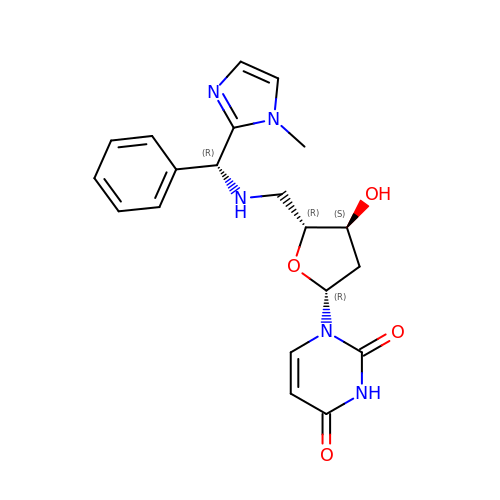2',5'-dideoxy-5'-{[(R)-(1-methyl-1H-imidazol-2-yl)(phenyl)methyl]amino}uridine | C20 H23 N5 O4 | KPWKGDCQLFIJMC-URHIDPGUSA-N> MGHHHHHHHHHHSSHIEGRHMESIEQQLTELRTTLRHHEYLYHVMDAPEIPDAEYDRLMRELRELETKHPELITPDSPTQRVGAAPLAAFSQIRHEVPMLSLDNVFDEESFLAFNKRVQDRLKNNEKVTWCCELMLDGLAVSILYENGVLVSAATRGDGTTGEDITSNVRTIRAIPLKLHGENIPARLEVRGEVFLPQAGFEKINEDARRTGGKVFANPRNAAAGSLRQLDPRITAKRPLTFFCYGVGVLEGGELPDTHLGRLLQFKKWGLPVSDRVTLCESAEEVLAFYHK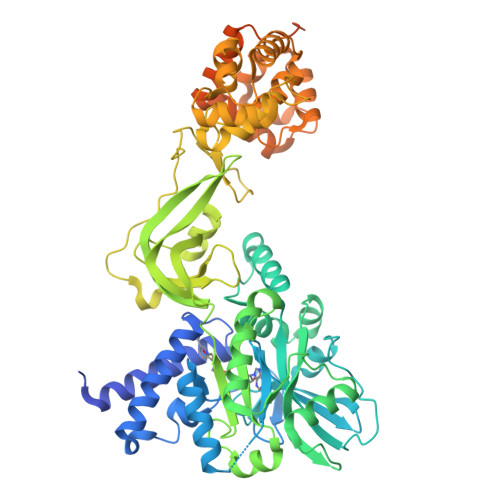VEEDRPTLGFDIDGVVIKVNSLAQQEQLGFVARAPRWAVAFKFPAQEQMTFVRDVEFQVGRTGAITPVARLEPVHVAGVLVSNATLHNADEIERLGLRIGDKVVIRRAGDVIPQVVNVVLSERPEDTREVVFPTHCPVCGSDVERVEGEAVARCTGGLICGAQRKESLKHFVSRRAMDVDGMGDKIIDQLVEKEYVHTPADLFKLTAGKLTGLERMGPKSAQNVVNALEKAKETTFARFLYALGIREVGEATAAGLAAYFGTLEALEAASIEELQKVPDVGIVVASHVHNFFAEESNRNVISELLAEGVHWPAPIVINAEEIDSPFAGKTVVLTGSLSQMSRDDAKARLVELGAKVAGSVSKKTDLVIAGEAAGSKLAKAQELGIEVIDEAEMLRLLGS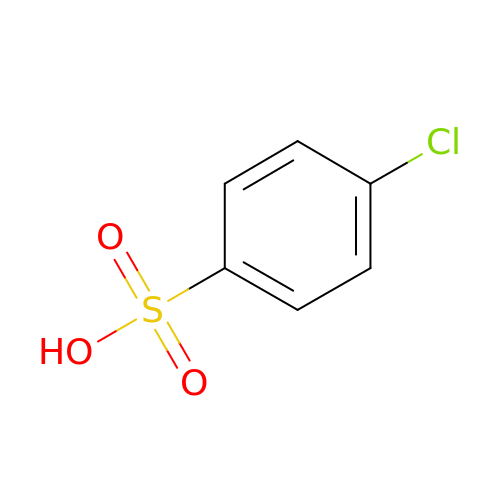4-chloranylbenzenesulfonic acid | C6 H5 Cl O3 S | RJWBTWIBUIGANW-UHFFFAOYSA-N>ETWWYNPSIVVHPHWREFDQVPDAVYYSLGIFIGICGIIGCGGNGIVIYLFTKTKSLQTPANMFIINLAFSDFTFSLVNGFPLMTISCFLKKWIFGFAACKVYGFIGGIFGFMSIMTMAMISIDRYNVIGRPMAASKKMSHRRAFIMIIFVWLWSVLWAIGPIFGWGAYTLEGVLCNCSFDYISRDSTTRSNILCMFILGFFGPILIIFFCYFNIVMSVSNHEKEMAAMAKRLNAKELRKAQAGANAEMRLAKISIVIVSQFLLSWSPYAVVALLAQFGPLEWVTPYAAQLPVMFAKASAIHNPMIYSVSHPKFREAISQTFPWVLTCCQFDDKETEDDKDAETEIPAGE[2x]

Rhodopsin is the primary photoreceptor molecule in the visual signaling cascade. The activation process of rhodopsin is initiated by the photo-isomerization of the retinal chromophore from the 11-cis to all-trans configuration. The primary photoreaction state (BATHO) relaxes thermally through lumirhodopsin (LUMI) to an activated state, META, which in turn stimulates the heterotrimeric G protein to activate the enzymatic cascade in photoreceptor cells. Indeed, bovine rhodopsin is hydrolyzed to free retinal and apoprotein after photo-activation, whereas the Meta state of squid rhodopsin is thermally stable. It is noteworthy that whereas signal transduction in vertebrate vision is mediated by the second messenger cyclic GMP, signal transduction in squid photoreceptor cells uses an inositol-1,4,5-trisphosphate signaling cascade in which photoactivated rhodopsin stimulates a Gq-type G protein.

In this study, we performed a crystallographic study of the LUMI state of squid rhodopsin to elucidate the essential structural change occurring in the activation process. From this spectral feature, it was suggested that the full conversion of BATHO to LUMI occurred at 170 K. Since META was scarcely formed at this temperature, the content of LUMI after crystal warming to 170 K was estimated to be 50%. In this study, diffraction data collected using a much lower flux of X-rays (6 × 1014 photons/mm2) were merged and the merged data were used for the structural analysis of LUMI. Although the C7 = C8 double bond and the adjacent bonds are largely twisted in BATHO, these bonds take on more relaxed configurations in LUMI. This relaxation is accompanied by a large movement of the central moiety of retinal towards the extracellular side. As a consequence, the retinal polyene chain in LUMI is sandwiched by the main chain of helix III and a β-strand in the E2 loop, as observed in RHOD (and ISO). Indeed, the all-trans retinal in LUMI is gently curved so as to embrace the indole ring of Trp274. The most significant difference between LUMI and RHOD is seen in the orientation of the C13 methyl group; i.e., it points toward helix VI in RHOD, whereas it points towards helix III in LUMI. This alteration is accompanied by reorientation of the Schiff base NH bond; i.e., it is directed towards Asn87 of helix II in RHOD, whereas it is re-orientated towards Asn185 in LUMI. A peculiar feature of the photoreaction of squid rhodopsin is seen in that the position/orientation of the β-ionone ring of retinal, which is tightly fixed by the surrounding aromatic residues, remains unaltered upon the formation of LUMI.>EVDPTHFEKRFLKRIRDLGEGHFGKVELCRYDPEGDNTGEQVAVKSLKPESGGNHIADLKKEIEILRNLYHENIVKYKG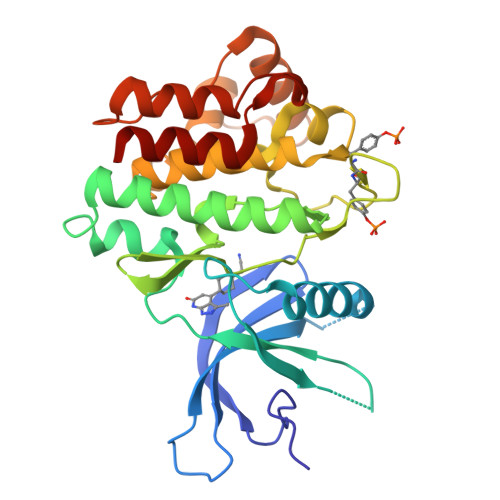ICTEDGGNGIKLIMEFLPSGSLKEYLPKNKNKINLKQQLKYAVQICKGMDYLGSRQYVHRDLAARNVLVESEHQVKIGDFGLTKAIETDKEYYTVKDDRDSPVFWYAPECLMQSKFYIASDVWSFGVTLHELLTYCDSDSSPMALFLKMIGPTHGQMTVTRLVNTLKEGKRLPCPPNCPDEVYQLMRKCWEFQPSNRTSFQNLIEGFEALLK[2x]>MHHHHHHGSKIKKIEPYVISHKLDTPFYFSQWQYDTRKICIVKITLDDGTYGWGEGYGPAAVIKSGIDFFTPFLLGKEAIGHEVLWQEMYRRSMDYARSGVLQAAISAIDVALWDIKGKLLNLPVSVLLGGVKNPIIEPYATGLYFTRTENLEELLVEEALLYKSQGFKATKMKVGLGIEQDLKYIAAIRKAIGPDMRLMIDSNHAYCYKEAIELARKAEKFDISWFEEPVSPEDYDGYKRLRQNTTIPISGGECEYLKYGFKRLFDKDCVDIAQPDICAAGGLTEVKKIATLAQTYNVDLVPHTWGTWIAISAAVHLVANLDKNPGRMYNDLPTMELDRTENALRDEVTLHKIKLENGHLEVPCTPGLGVDVDMDKLEHYLDKEIHKDGATKIRS[8x]

Carrageenans, alongside agars, are the main cell wall polysaccharides of red macroalgae and play vital roles in the development and physiology of these photosynthetic eukaryotes. In marine ecosystems carrageenans constitute a huge biomass and thus a precious carbon source for marine heterotrophic bacteria (MHB). The marine Bacteroidetes Zobellia galactanivorans DsijT, originally isolated from a healthy red macroalga, is a bacterial model for the bioconversion of algal polysaccharides. Here we describe in Z. galactanivorans the discovery and the integrative characterization of the complete pathway for utilization of the kappa family carrageenans (containing 3,6-anhydro-d-galactose units, mainly kappa-, iota- and beta-carrageenans), which is carried out by a complex regulon including a dedicated atypical PUL, lacking the susCD-like pair, and carrageenan-induced loner genes including distal susCD-like pairs.

The resulting 3,6-anhydro-d-galactonate is converted to 2-keto-3-deoxy-d-galactonate by ZGAL_3156, as measured through the thiobarbituric acid (TBA) assay. ZGAL_3156 did not demonstrate any activity on D-AnG alone and is thus a 3,6-anhydro-d-galactonate cycloisomerase (dauB). The crystal structure reveals an octamer, not uncommon in the enolase superfamily. A size-exclusion column analysis confirmed that ZGAL_3156 constitutes an octamer in solution. In the enolase superfamily, the active site is located at the interface of the two domains, the lid domain shielding the catalytic machinery from bulk solvent. Two disordered regions (17–26 and 138–143) were not modeled. They are close spatially and constitute the tip of the lid domain. The residues involved in the coordination of the catalytic cation (Asp194, Glu220, and Glu246) and the predicted general base (Lys166) and acid (His296) of AtGCI are strictly conserved between AtGCI and ZGAL_3156 and have similar spatial orientations. This cation was modeled as an Mg2+ in ZGAL_3156 and as a Ca2+ in AtGCI. The residues shaping the substrate-binding pocket in AtGCI originate from the TIM-barrel and the lid domain of one monomer and from the loop between helices α2 and α3 of the neighboring monomer.> QGENISSLLRELYAKP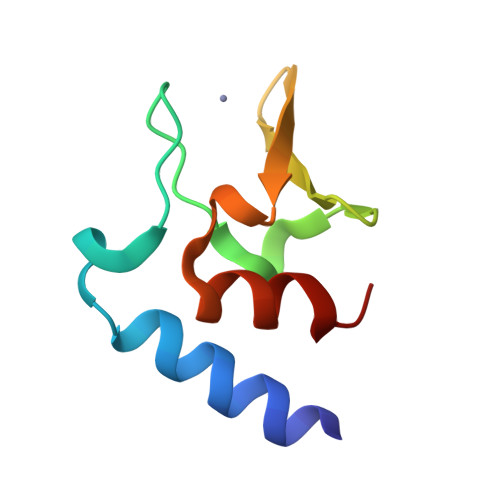LSERHVESDGLIFDPAQITSRTANGVAVPHGDHYHFIPYSQLSPLEEKLARIIPL(6R,8S,9S)-8-(hydroxymethyl)-6,11,11-tris(oxidanyl)-9-propyl-dodecanoic 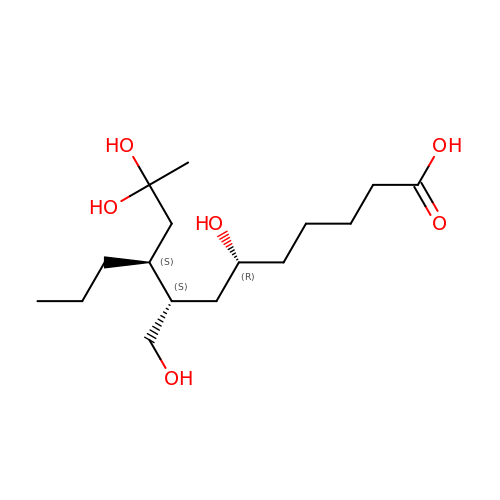acid | C16 H32 O6 | XPIGONIHXZGSPX-BFHYXJOUSA-N> MPTLTARSVIPPYMLRRIIEHGSLPQRDCALHTLNHVQSLLGNKPLRAPGAKTSTGGEVIRDIYDAENSTQLPGKQVRNEGQASNHDVAVDEAYDYLGVTYDFFWQAFKRNSLDNQGLPLTGSVHYGKEYQNAFWNGQQMV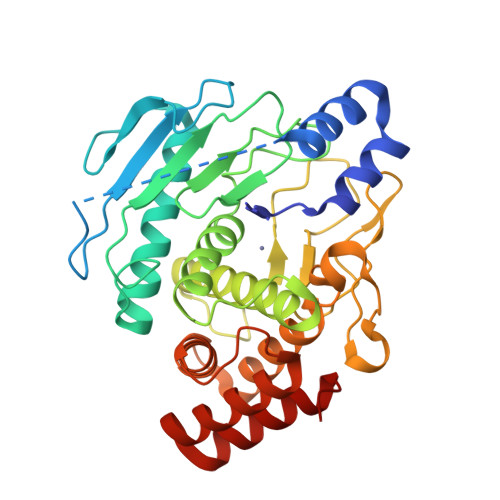FGDGDGEIFNRFTIAIDVVGHALAHGVTESEAGLIYFQQAGALNESLSDVFGSLVKQFHLKQTADKADWLIGEGLLAKGINGKGLRSMSAPGTAYDDPLLGKDPQPASMKDYIQTKEDNGGVHLNSGIPNRAFYLAATALGGYAWEKAGYIWYDTLCDKALPQDADFATFARTTVKHAEQRFDSKVAQKVQQAWHQVGVA> MSEAYFRVESGALGPEENFLSLDDILMSHEKLPVRTETAMPRLGAFFLERSAGAETDNAVPQGSKLELPLWLAKGLFDNKRRILSVELPKIYQEGWRTVFSA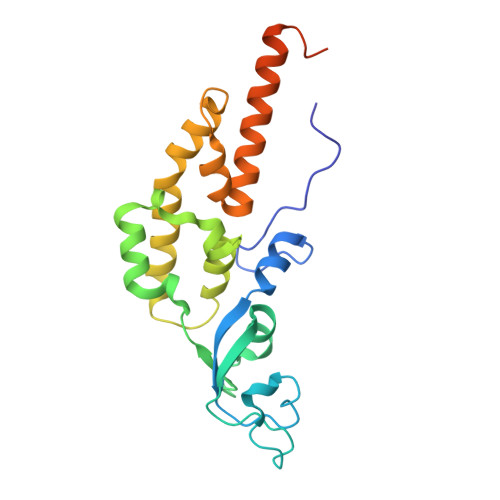DPNVVDLHKMGPHFYGFGSQLLHFDSPENADISQSLLQTFIGRFRRIMDSSQNAYNEDTSALVARLDEMERGLFQTGQKGLNDFQCWEKGQASQITASNLVQNYKKRKFTDMED>MVKVDLESKRYGEKLKEVFLMLDNNVVECIKEITESSRNGKLVFFVGAGVSTLSDYPQWWRLVDKYHEELYGSPKKGNYSSDEYLRIPQIFYNVKGEMAFDGILKDFFQVDKPTNPIHDKILAMNPAHVITTNYDNLIDTACWKRGKYFSVISAEEDVANATSSRYLLKVAGDFRKGFKGENVVLKEDDYLNYDQNYPLISNLMKTIIATHTIVFIGYGLGDYNINMLLNWVRKLQKDSFHKPFFIRTDPSPIENETLIYYENKGLRIIDAASLIDSNEYDYLERYSAVMDLLIESQENKFITKDDEVIDYIYGKISPLFALQYIRKIDLKHVFEYDYHFEVNGTVVRHKNKGFGYMERFFELKESCDERSKLSKKQYERFNALFNFFEKNGVICMAKDAGTLNTSIEINSLAYHGKYDVMKKFIEEQSVSIEDDYKKAFFLACLGRWEESYDLYSNIILNSIDESNGCVYYLSQINRYRIYQSITQAVTQFNGLGLLTFGRHYKPFTDEFLARIEREMTNFNIDDLFNGMPFEFQKKYKILEFLSDNQFLYDDTVKLFELTNKVRSEMSEGSYSFGMSSDIVVL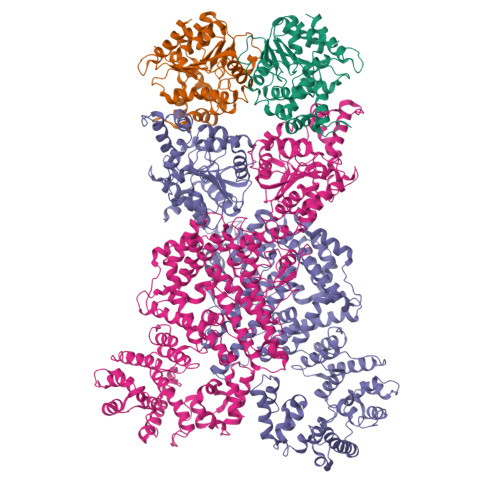LRLYDNLRFLYENCLWSVSFHEFHQYIRNSMSLLIEKAEYERTRDIDELGFSFFGKKSGFFMEYYDFVNISRHFKIDDIKNLERSCSIDKIRFGEQEKIEEYLVGIAEEITKQFSANGMNVVFYTQFISEAKAALYFAKYVKLSEEGLGKIVKALLFYFPERDLDIGKRYVWLERLTKCNELPKSIISIIDDFLVLQAEKHIDQNYSEVSSNGLYSRDYGALIKHFEKNFISKRLSEITLCLTQDKQKQIDFLFKLLPLLSTNAKSHLLSFKSVENINDLMNGIRIGLIDEFTPEHEELIIEYLETRKVNYIVEKEKGIQTFSSNDYMSTFGIWYFLEEINNSKMEEFIGMDDQYDFFVDPENFDYKKFIPSWLKNYNDKLLGKIAGNKHMKHHVIEVLKERVKNSNDKRYLEILMNYFI[4x]> GAENNM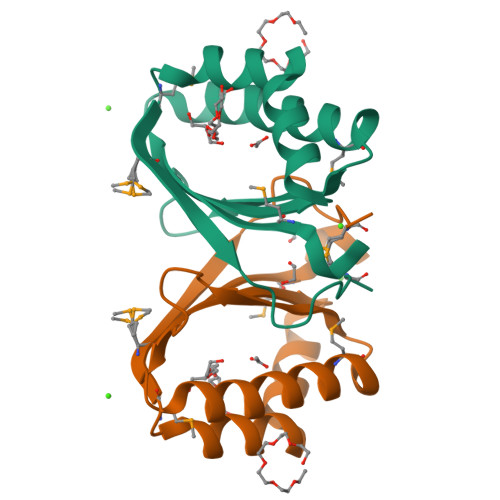VRLSRIIIDPERLEEYNAYLKEEIEVSMRLEPGVLVLYAVAEKERPNHVTILEIYADEAAYKSHIATPHFKKYKEGTLDMVQMLELIDATPLIPGLKMK>[6x]CEEPPTFEAMELIGKPKPYYEIGERVDYKCKKGYFYIPPLATHTICDRNHTWLPVSDDACYRETCPYIRDPLNGQAVPANGTYEFGYQMHFICNEGYYLIGEEILYCELKGSVAIWSGKPP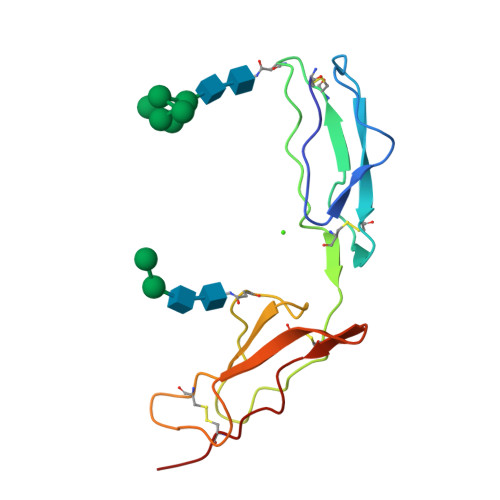ICEKV6-chloro-N-{(3S)-1-[(2S)-1-(morpholin-4-yl)-1-oxopropan-2-yl]-2-oxo-2,3-dihydro-1H-pyrrol-3-yl}-N-(2-oxobutyl)naphthalene-2-sulfonamide 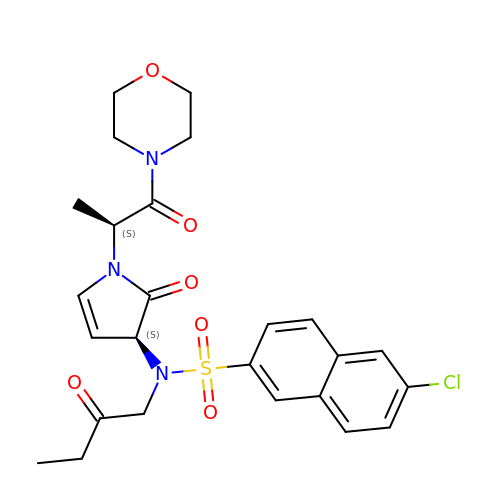| C25 H28 Cl N3 O6 S | MPHFQCQENHLINH-SBUREZEXSA-N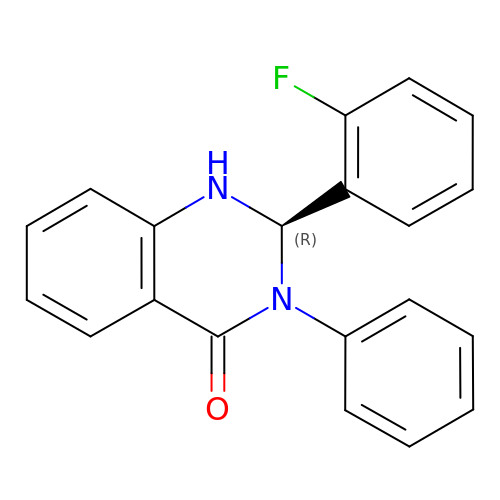(2R)-2-(2-fluorophenyl)-3-phenyl-1,2-dihydroquinazolin-4-one | C20 H15 F N2 O | UMMDFHVNOCVOCD-LJQANCHMSA-N>GSHMRHVEHTVTVAAPADLVWEVLADVLGYADIFPPTEKVEILEEGQGYQVVRLHVDVAGEINTWTSRRDLDPARRVIAYRQLETAPIVGHMSGEWRAFTLDAERTQLVLTHDFVTRAAGDDGLVAGKLTPDEA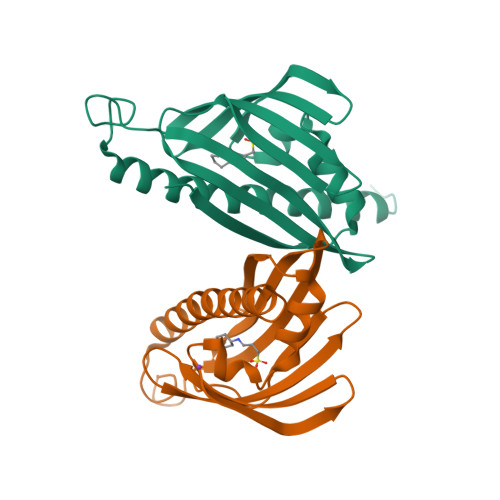REMLEAVVERNSVADLNAVLGEAERRVRAAGGVGTVTA[6x]>MAKLIAESGSTKTEWSLVEGEHLIQRVFTEGLNPFFQTRREISRSIRLGLPDSFFKRKLEQVFFYGAGCTSAEKKSVVEASLVAQFKTPAYVESDLLAAARGLFQHDSGIACILGTGSNSCFYDGHVIVKNVRAGGYILGDEGSGAALGKQFLSDVLKKLAPQVLIDDFFEKYDLTPHDVMDVVYNRPFPNRFLAEQSCFLADYLRLDYVKGLLLSNLRSFFLRNVMQYDYLNYPIRFVGSVAYNYADLLHQVGKEFGVELSVVEETPMGGLIKYHAFPPDDPESLEHHHHHH[6x]

Unlike other bacteria, the pathogenic Tannerella forsythia, a member of the red complex group of bacteria associated with the late stages of periodontitis, lacks biosynthetic pathways for MurNAc production and therefore obtains MurNAc from the environment. Sugar kinases play a crucial role in the MurNAc recycling process, activating the sugar molecules by phosphorylation. MurK and K1058 are two sugar kinases of the cell wall recycling system of T. forsythia, sharing a sequence identity of 44% and separated by a single PGN-scavenging operon within the genome. Structural and sequence data showed that MurK and K1058 both belong to the group of ribonuclease H-like kinases and are members of the ASKHA (acetate and sugar kinase/hsc70/actin) superfamily.

The production of MurNAc-bound crystals of MurK and K1058 was very challenging but eventually yielded crystals of MurK and K1058 in complex MurNAc (termed MurK/MurNAc and K1058/MurNAc, respectively). Both crystal forms diffract to approximately 3 Å resolution and contain six protomers in the ASU corresponding to three biological dimers. An in-depth active site comparison of both MurNAc-liganded structures showed a very similar binding of MurNAc as in MurK, with the sugar molecule slightly tilted around the bond between O1 and C5. When comparing all residues of the sugar-binding site, differences can be found in two locations. Firstly, residue I69 of MurK is replaced by a less bulky and more polar threonine (T69) in K1058. Secondly, in the region involved in lactyl ether recognition, residues S133 and P134 are substituted by an arginine and an alanine, respectively. All other residues in the MurNAc-binding site are identical and occupy conformations very close to MurK. Moreover, R132 in K1058 seems to be an optimal candidate to bind MurNAc via its carboxy group. Although we do not observe such an interaction, probably because the side chain conformation would have to be in an “bent back” setup, a partial charge compensation is possible, which might compensate for the loss in affinity by the loss of water-mediated hydrogen bonding to S133 in MurK. Indeed, the affinity for K1058 is higher than MurK, with an apparent KM value of 28 ± 10 μM, but the catalytic turnover is severely reduced and suggests that MurNAc might not be the natural substrate of K1058.2-{[FORMYL(HYDROXY)AMINO]METHYL}-4-METHYLPENTANOIC 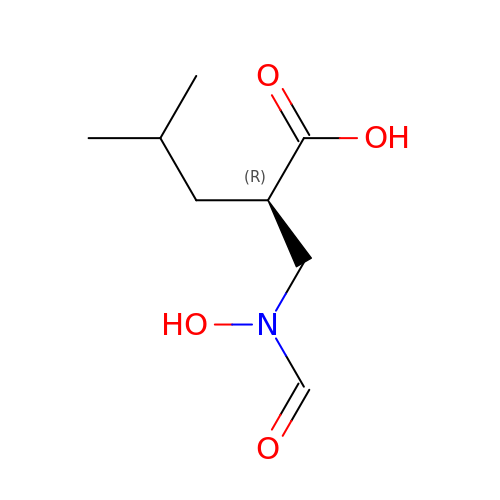ACID | C8 H15 N O4 | LFMOJNDZFCHHPV-SSDOTTSWSA-N N-{6-[6-amino-5-(trifluoromethyl)pyridin-3-yl]imidazo[1,2-a]pyridin-2-yl}acetamide | C15 H12 F3 N5 O | 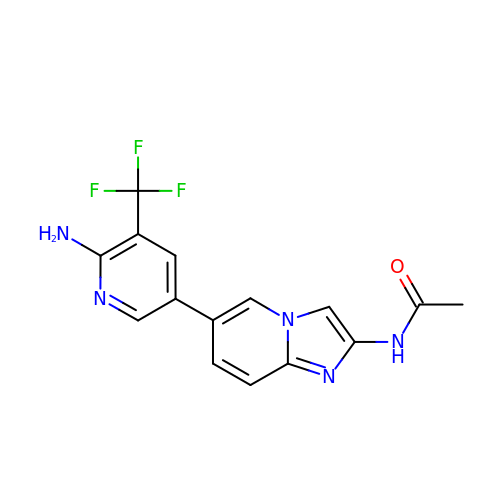TVUPSIBSWDXJGQ-UHFFFAOYSA-N>LPTTHEVHVYGSINGVEFDLVGSGKGNPKDGSEEIQVKSTKGPLGFSPYIVVPNIGYGFHQYLPFPDGMSPFQAAADDGSGYVVHRTIQFEDGASLTGNYRYSYDGGHIKGEFHVVGSGFPADGPVMTKSLTAVDWSVATMLFPNDTTVVSTIDWTCPTTSGKRYHATLRTNYTFAKPIA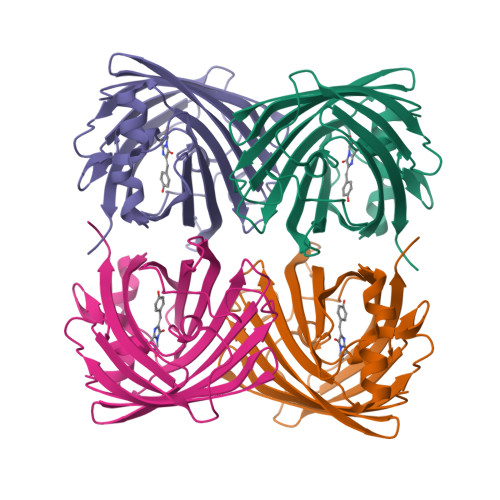ATILQKQPMFVFRKTEVKASDAEINLKEWQKAFHDL[8x]> SSQIRQNYSTEVEAAVNRLVNLYLRASYTYLSLGFYFDRDDVALEGVCHFFRELAEEKREGAERLLKMQNQRGGRALFQDLQKPSQDEW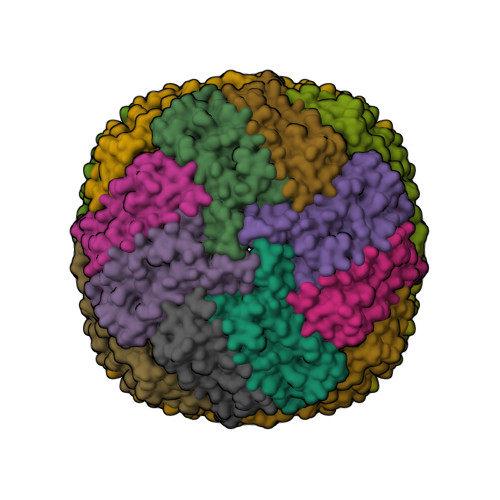GTTLDAMKAAIVLEKSLNQALLDLHALGSAQADPHLCDFLESHFLDEEVKLIKKMGDHLTNIQRLVGSQAGLGEYLFECCTLKHD>[4x]GPMSRNDKEPFFVKFLKSSDNSKCFFKALESIKEFQSEEYLQIITEEEALKIKENDRSLYICDPFSGVVFDHLKKLGCRIVGPQVVIFCMHHQRCVPRAEHPVYNMVMSDVTISCTSLEKEKREEVHKYVQMMGGRVYRDLNVSVTHLIAGE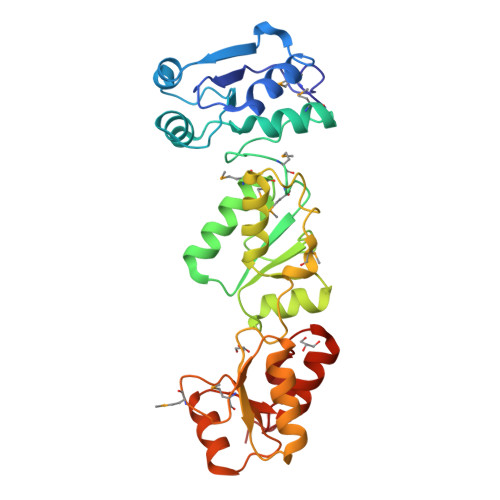VGSKKYLVAANLKKPILLPSWIKTLWEKSQEKKITRYTDINMEDFKCPIFLGCIICVTGLCGLDRKEVQQLTVKHGGQYMGQLKMNECTHLIVQEPKGQKYECAKRWNVHCVTTQWFFDSIEKGFCQDESIYKTEPRPEA> Y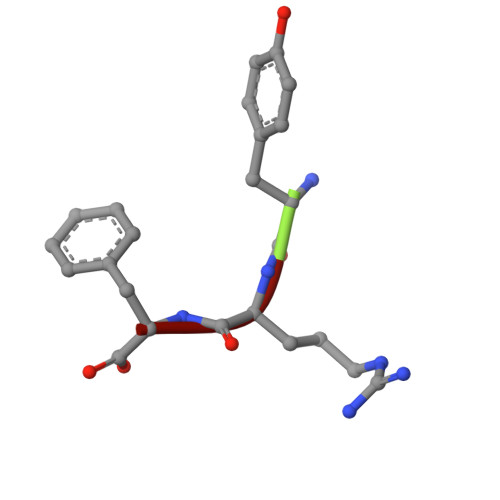RF> GSAMAIVSMECKTIVSQYGEMIWDLLVSGVRPDQVCSQAGLCFVDGAQHVSSNIKTVVERETEGSSVGEAPLCTACEMAVVWMQNQLKQEGTKEKVLEYVNQLCE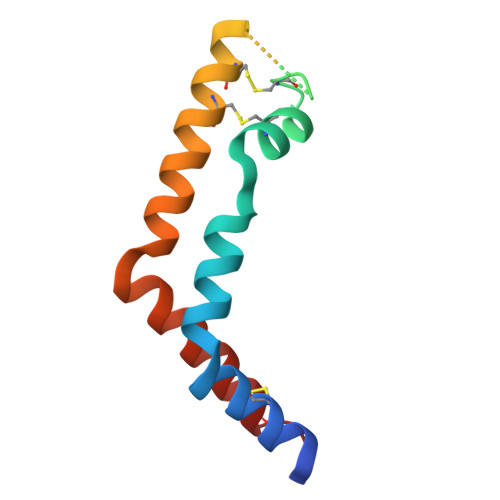KIP> VPRGSH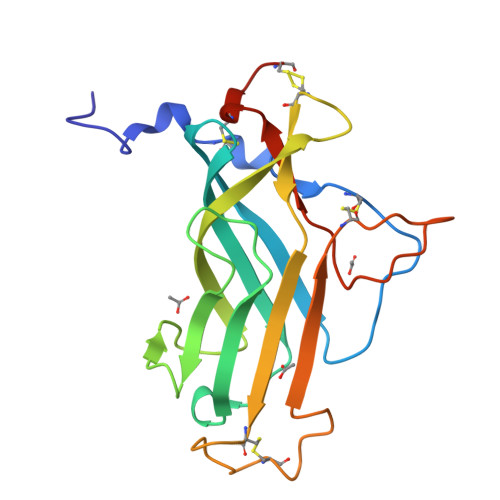MSSGKTCPTSEVSPACYANQWETTFPPSDIKITGATWVQDNIYDVTLSYEAESLELENLTELKIIGLNSPTGGTKLVWSLNSKVYDIDNPAKWTTTLRVYTKSSADDCYVEMYPFQIQVDWCEAGASTDGCSAWKWPKSYDYDIGCDNMQDGVSRKHHPVYKWPKKCSSNCGVEPTT>[4x]SHMSGLKPCVDWLQVTFKTGQDSVKKCVEKLEKVFEILGLNEAEFLPLKNGKYGYKQGVAFQGNPVLAVYYDGADDMGIHVEMTGQGCRLFELHTSINWYELFYRLVYEYEVNITRLDVAVDDFKGYFKINTLVKKLKDDEVTSRFKKARHI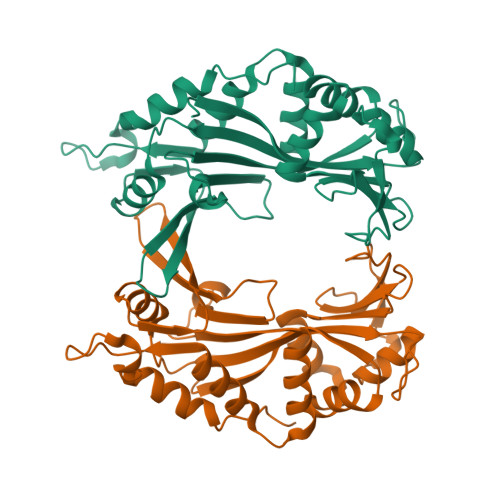ENIVIEGGETIGHTLYFGAPSSDIQVRFYEKNVQMGMDIDVWNRTEIQLRDDRAHVVAQIIADDVLPLGEIVAGLLRNYIQFRTRKATDKNKKRWPLARFWLNFLGDVQPLRIAKQMPK>[2x]SQKFDVIVIGAGPGGYVAAIKSAQLGLKTALIEKYKGKEGKTALGGTCLNVGCIP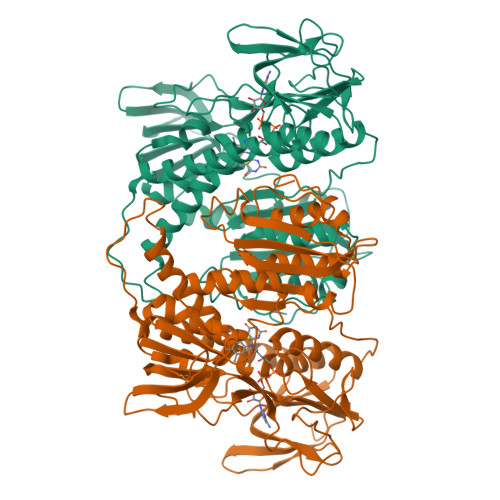SKALLDSSYKFHEAHESFKLHGISTGEVAIDVPTMIARKDQIVRNLTGGVASLIKANGVTLFEGHGKLLAGKKVEVTAADGSSQVLDTENVILASGSKPVEIPPAPVDQDVIVDSTGALDFQNVPGKLGVIGAGVIGLELGSVWARLGAEVTVLEAMDKFLPAVDEQVAKEAQKILTKQGLKILLGARVTGTEVKNKQVTVKFVDAEGEKSQAFDKLIVAVGRRPVTTDLLAADSGVTLDERGFIYVDDYCATSVPGVYAIGDVVRGAMLAHKASEEGVVVAERIAGHKAQMNYDLIPAVIYTHPEIAGVGKTEQALKAEGVAINVGVFPFAASGRAMAANDTAGFVKVIADAKTDRVLGVHVIGPSAAELVQQGAIAMEFGTSAEDLGMMVFAHPALSEALHEAALAVSGHAIHVANRKK> GEFSGPPVERCGVLSKWTNYIHGWQDRWVVLKNNALSYYKSEDETEYGCRGSICL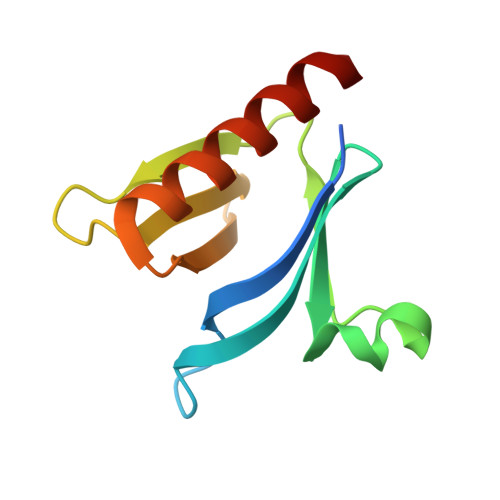SKAVITPHDFDECRFDISVNDSVWYLRAQDPDHRQQWIDAIEQHKTESGYG> SGISLDNSYKMDYPEMGLCIIINNKNFHKST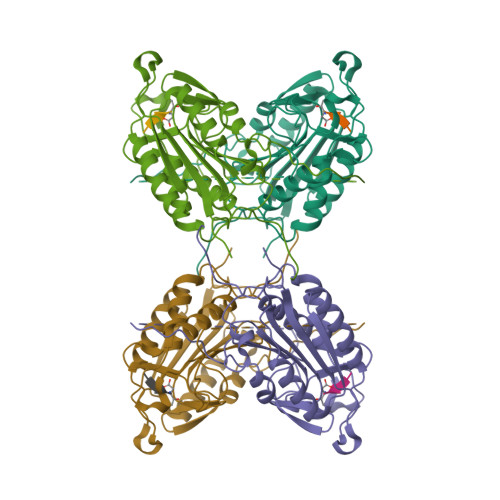GMTSRSGTDVDAANLRETFRNLKYEVRNKNDLTREEIVELMRDVSKEDHSKRSSFVCVLLSHGEEGIIFGTNGPVDLKKITNFFRGDRCRSLTGKPKLFIIQACRGTELDCGIETDSGVDDDMACHKIPVEADFLYAYSTAPGYYSWRNSKDGSWFIQSLCAMLKQYADKLEFMHILTRVNRKVATEFESFSFDATFHAKKQIPCIVSMLTKELYFYHH>[4x]KVTLPDLK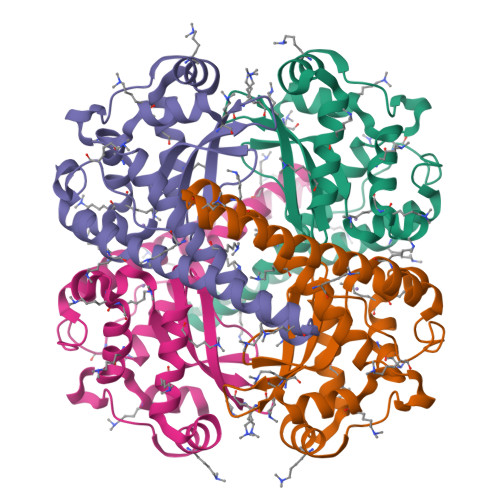WDFGALEPYISGQINELHYTKHHQTFVNGFNTAVDQFQELSDLLAKEPSPANARKMIAIQQNIKFHGGGFTNHCLFWENLAPESQGGGEPPTGALAKAIDEQFGSLDELIKLTNTKLAGVQGSGWAFIVKNLSNGGKLDVVQTYNQDTVTGPLVPLVAIDAWEHAYYLQYQNKKADYFKAIWNVVNWKEASRRFDAGKI tert-butyl 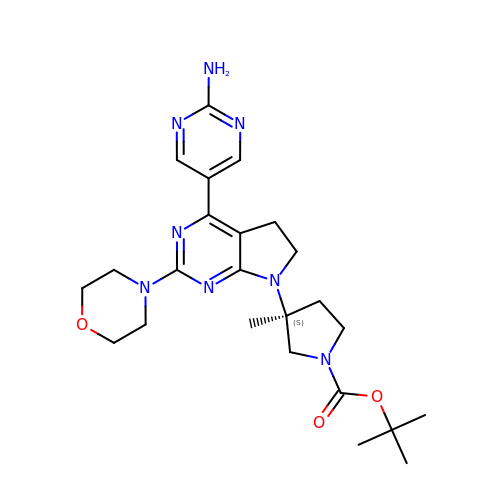(3S)-3-[4-(2-aminopyrimidin-5-yl)-2-(morpholin-4-yl)-5,6-dihydro-7H-pyrrolo[2,3-d]pyrimidin-7-yl]-3-methylpyrrolidine-1-carboxylate | C24 H34 N8 O3 | MEWKDLGRKBRJAF-DEOSSOPVSA-N>[2x]YFGKLESKLSVIRNLNDQVLFIDQGNRPLFEDMTDSDCRDNAPRTIFIISMYKDSQPRGMAVTISVACAAASTLSCENKIISFKEMNPPDNIKD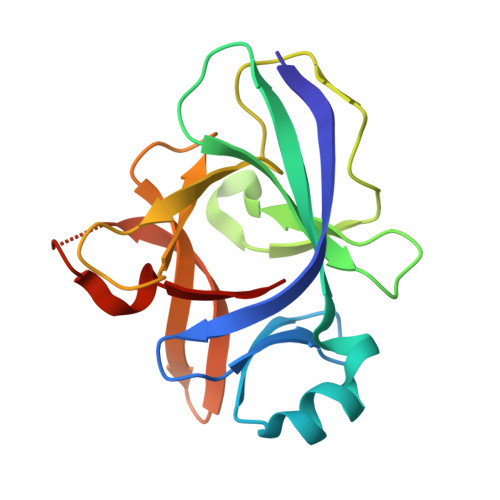TKSDIIFFQRSVPGHDNKMQFESSSYEGYFLACEKERDLFKLILKKEDELGDRSIMFTVQNED[(1R)-3-(4-chlorophenyl)-3-oxo-1-phenylpropyl]propanedioic acid | C18 H15 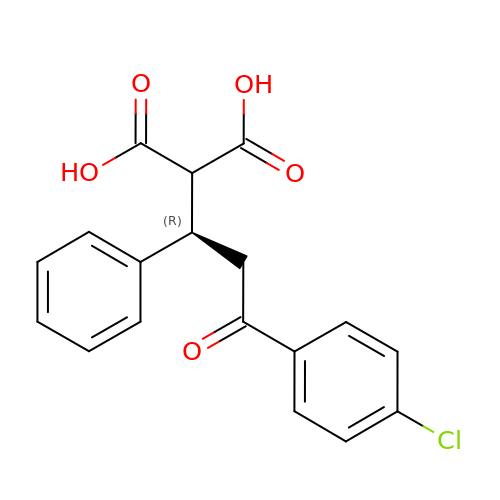Cl O5 | XOOQYQRTMFAOAP-AWEZNQCLSA-N> AEIYNKDGNKVDLYGKAVGLHYFSKGNGENSYGGNGDMTYARLGFKGETQINSDLTGYGQWEYNFQGNNSEGADAQTGNKTRLAFAGLKYADVGSFDYGRNYGVVYDALGYTGMLPEFGGDTAYSDDFFVGRVGGVATYRNSNFFGLVDGLNFAVQYLGKNERDTARRSNGDGVGGSISYEYEGFGIVGAYGAADRTNLQEAQPLGNGKKAEQWATGLKY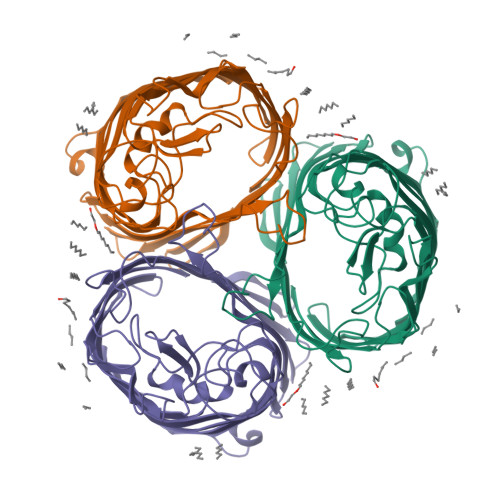DANNIYLAANYGETRNATPITNKFTNTSGFANKTQDVLLVAQYQFDFGLRPSIAYTKSKAKDVEGIGDVDLVNYFEVGATYYFNKNMSTYVDYIINQIDSDNKLGVGSDDTVAVGIVYQF> MSGFHNVGNINMMAQQQMQQNRIKISVRNWQNATMNDLINFISRNARVAVYDAHVEGPLVIGYVNSKAEAESLMKWNGVRFAGSNLKFELLDNNGASAGTSDTISFLRGVLLKRYDPQTKLLNL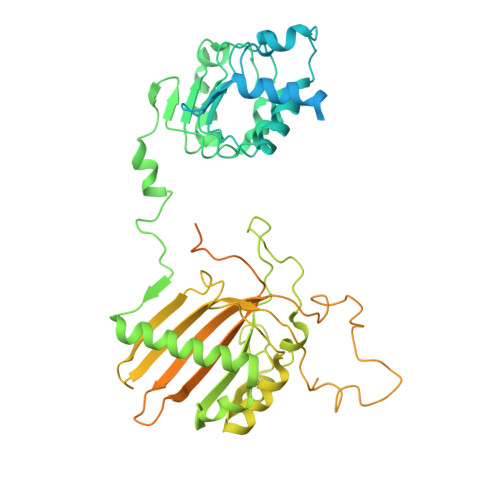GALHSDPELIQKGVFSSISTQSKMFPAMMKLASTEKSLIVESVNLADNQLKDISAISTLAQTFPNLKNLCLANNQIFRFRSLEVWKNKFKDLRELLMTNNPITTDKLYRTEMLRLFPKLVVLDNVIVRDEQKLQTVYSLPMKIQQFFFENDALGQSSTDFATNFLNLWDNNREQLLNLYSPQSQFSVSVDSTIPPSTVTDSDQTPAFGYYMSSSRNISKVSSEKSIQQRLSIGQESINSIFKTLPKTKHHLQEQPNEYSMETISYPQINGFVITLHGFFEETGKPELESNKKTGKNNYQKNRRYNHGYNSTSNNKLSKKSFDRTWVIVPMNNSVIIASDLLTVRAYSTGAWKTASIAIAQPPQQQASVLPQVASMNPNITTPPQPQPSVVPGGMSIPGAPQGAMVMAPTLQLPPDVQSRLNPVQLELLNKLHLETKLNAEYTFMLAEQSNWNYEVAIKGFQSSMNGIPREAFVQF> GAMGPQEYTLIKLKIHLIPEFLGSIVKGREVFVVCATLRPETMYGQTNCWILPDGEYDLVLAFDQVIPYDAKTSEGVLCKIFDKYEDTMKECNTVYICSERSAYNMAYQGIVPLIHGREQGVSDKLLPRIVSLGKVYGEQLIGTPLSAPMTPYSLIFILPMFSISMEKGTGIVTSVPSDSPDDYAALRDIKTKPLLREKYSIKDEWILDPLEIIEVPGFGFMTAELLCNQYKIQSQNDSAKLKQAKEEIYKKEFYEGILIRGKYSGMKICDAKELIRESLI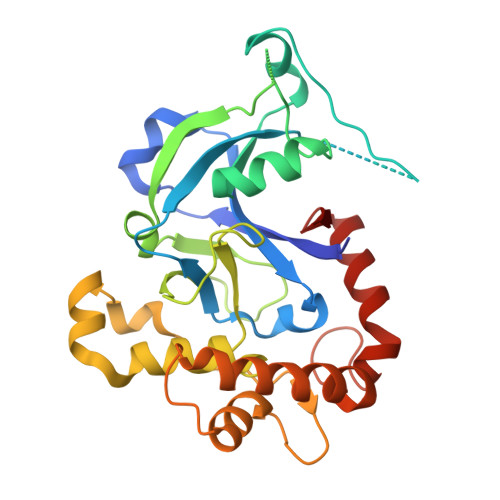KDGYALIYLE> VVGGLVALRGAHPYIAALYWGHSFCAGSLIAPCWVLTAAHCLQDRPAPEDLTVVLGQERRNHSCEPCQTLAVRSYRLHEAFSPVSYQHDLALLRLQEDADGSCALLSPYVQPVCLPSGAAR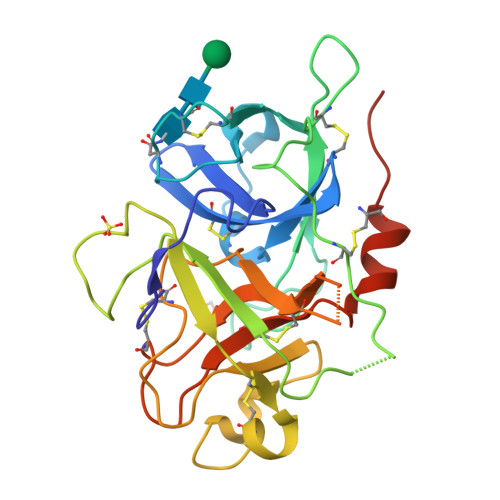PSETTLCQVAGWGHQFEGAEEYASFLQEAQVPFLSLERCSAPDVHGSSILPGMLCAGFLEGGTDACQGDSGGPLVCEDQAAERRLTLQGIISWGSGCGDRNKPGVYTDVAYYLAWIREHTVSTRTGHHHHHH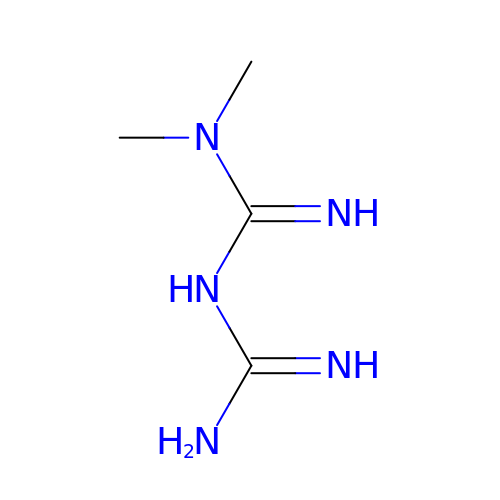Metformin | C4 H11 N5 | XZWYZXLIPXDOLR-UHFFFAOYSA-N>MERPQPDSMPQDLSEALKEATKEVHTQAENAEFMRNFQKGQVTRDGFKLVMA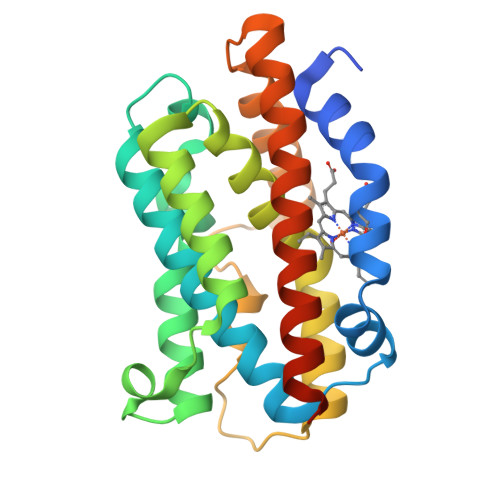SLYHIYVALEEEIERNKESPVFAPVYFPEELHRKAALEQDLAFWYGPRWQEVIPYTPAMQRYVKRLHEVGRTEPELLVAHAYTRYLADLSGGQVLKKIAQKALDLPSSGEGLAFFTFPNIASATKFKQLYRSRMNSLEMTPAVRQRVIEEAKTAFLLNIQLFEELQELLTHDTKDQSPSRA[2x]>[4x]MPLNRTLEMSELPGLEDWEDEFDLENAVLFEVAWEVANKVGGIYTVLQTKAKVTGDEWGDNYFLVGPYTEQGVRTQVELLEAPTPALKRTLDSMNSK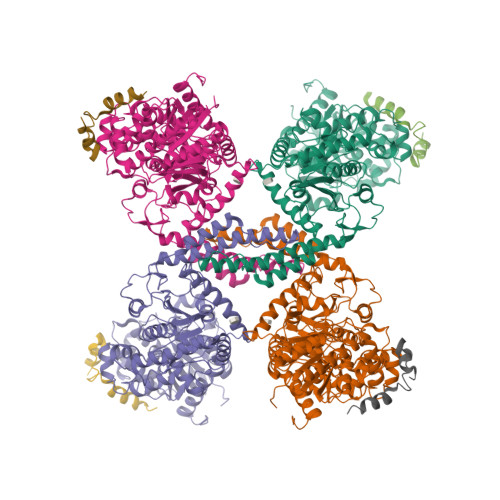GCKVYFGRWLIEGGPLVVLLDVGASAWALERWKGELWDTCNIGVPWYDREANDAVLFGFLTTWFLGEFLAQSEEKPHVVAHFHEWLAGVGLCLCRARRLPVATIFTTHATLLGRYLCAGAVDFYNNLENFNVDKEAGERQIYHRYCMERAAAHCAHVFTTVSQITAIEAQHLLKRKPDIVTPNGLNVKKFSAMHEFQNLHAQSKARIQEFVRGHFYGHLDFNLDKTLYFFIAGRYEFSNKGADVFLEALARLNYLLRVNGSEQTVVAFFIMPARTNNFNVETLKGQAVRKQLWDTANTVKEKFGRKLYESLLVGSLPDMNKMLDKEDFTMMKRAIFATQRQSFPPVCTHNMLDDSSDPILTTIRRIGLFNSSADRVKVIFHPEFLSSTSPLLPVDYEEFVRGCHLGVFPSYYEPWGYTPAECTVMGIPSISTNLSGFGCFMEEHIADPSAYGIYILDRRFRSLDDSCSQLTSFLYSFCQQSRRQRIIQRNRTERLSDLLDWKYLGRYYMSARHMALSKAFPEHFTYEPNEADAAQGY;>GPMTDQAFVTLTTNDAYAKGALVLGSSLKQHRTTRRLVVLATPQVSDSMRKVLETVFDEVIMVDVLDSGDSAHLTLMKRPELGVTLTKLHCWSLTQYSKCVFMDADTLVLANIDDLFDREELSAAPDPGWPDCFNSGVFVYQPSVETYNQLLHLASEQGSFDGGDQGILNTFFSSWATTDIRKHLPFIYNLSSISIFSYLPAFKVFGASAKVVHFLGRVKPWNYTYDPKTKSVKSEAHDPNMTHPEFLILWWNIFTTNVLPLLQQFGLVKDTCSYVNVLSDLVYTLAFSCGFCRKEDVSGAISHLSLGEIPAMAQPFVSSEERKERWEQGQADYMGADSFDNIKRKLDTYLQ[4x]Reverse transcriptase (RT) of human immunodeficiency virus (HIV) is essential for viral replication due to its responsibility for the conversion of viral RNA genome into DNA. Thus, RT represents an important and established target among anti-HIV-1 therapies to treat acquired immune deficiency syndrome. RT contains two distinct druggable sites: the polymerase catalytic site that is available for nucleoside reverse transcriptase inhibitors (NRTIs) and their acyclic nucleoside phosphonate analogues (ANPs), and the allosteric binding site available for non-NRTIs (NNRTIs). NNRTIs target an allosteric binding pocket which is situated about 10 Å from the polymerase catalytic site. HIV-1 RT was co-crystallized with cyanovinyl compounds 2, 4, and 6 to determine the effect of the size of ring B on binding in the NNRTI pocket.

All three compounds maintain a hydrogen bond between the aniline nitrogen and the K101 backbone carbonyl. The potential for a second hydrogen bond between the pyrimidine core nitrogen and the K101 backbone nitrogen varies between structures. This distance is longest with the five-membered ring at 3.4 Å, suggesting that it likely does not contribute significantly to binding affinity. Due to an opening and solvent-accessible area around the core, there is water observed interacting with ring B in the five- and six-membered structures of compounds 2 and 4, but not with the seven-membered ring B of compound 6. The co-crystal structure with compound 2 shows the most dramatic change in protein conformation. Notably, the side chain of Y188 rotates away from Y181 and sits more parallel to the cyanovinyl. To allow this shift, sheets β9 and β10 move, resulting in the Cα atom of D185 moving 4.7 Å compared to the RPV bound structure. Because of this, several amino acid residues become disordered at the periphery of the pocket, markedly from residues 217 to 222. These protein movements are possibly due to the position of the carbonyl in ring B and/or the wider distance between the arms in the horseshoe shape. Most importantly, compound 2 exhibited significantly improved phosphate-buffered saline solubility (10.4 μM) compared to ETV and RPV (≪1 μM).

> PISPIETVPVKLKPGMDGPKVKQWPLTEEKIKALVEICTEMEKEGKISKIGPENPYNTPVFAIKKKDSTKWRKLVDFRELNKRTQDFWEVQLGIPHPAGLKKKKSVTVLDVGDAYFSVPLDEDFRKYTAFTIPSINNETPGIRYQYNVLPQGWKGSPAIFQSSMTKILEPFRKQNPDIVIYQYMDDLYVGSDLEIGQHRTKIEELRQHLLRWGLTTPDKKHQKEPPFLWMGYELHPDKWTVQPIVLPEKDSWTVNDIQKLVGKLNWASQIYPGIKVRQLCKLLRGTKALTEVIPLTEEAELELAENREILKEPVHGVYYDPSKDLIAEIQKQGQGQWTYQIYQEPFKNLKTGKYARMRGAHTNDVKQLTEAVQKITTESIVIWGKTPKFKLPIQKETWETWWTEYWQATWIPEWEFVNTPPLVKLWYQLEKEPIVGAETFYVDGAANRETKLGKAGYVTNRGRQKVVTLTDTTNQKTELQAIYLALQDSGLEVNIVTDSQYALGIIQAQPDQSESELVNQIIEQLIKKEKVYLAWVPAHKGIGGNEQVDKLVSAGIRKVL;> PISPIETVPVKLKPGMDGPKVKQWPLTEEKIKALVEICTEMEKEGKISKIGPENPYNTPVFAIKKKDSTKWRKLVDFRELNKRTQDFWEVQLGIPHPAGLKKKKSVTVLDVGDAYFSVPLDEDFRKYTAFTIPSINNETPGIRYQYNVLPQGWKGSPAIFQSSMTKILEPFRKQNPDIVIYQYMDDLYVGSDLEIGQHRTKIEELRQHLLRWGLTTPDKKHQKEPPFLWMGYELHPDKWTVQPIVLPEKDSWTVNDIQKLVGKLNWASQIYPGIKVRQLCKLLRGTKALTEVIPLTEEAELELAENREILKEPVHGVYYDPSKDLIAEIQKQGQGQWTYQIYQEPFKNLKTGKYARMRGAHTNDVKQLTEAVQKITTESIVIWGKTPKFKLPIQKETWETWWTEYWQATWIPEWEFVNTPPLVKLWYQLEKEPIVGAETF>GPSEGIVPGPPTDLSVTEATRSYVVLSWKPPGQRGHEGIMYFVEKCEAGTENWQRVNTELPVKSPRFALFDLAEGKSYCF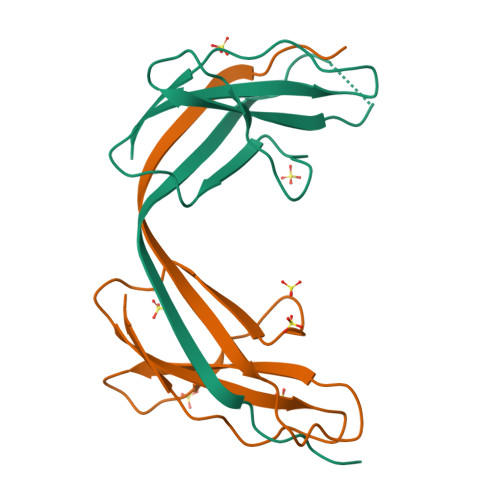RVRCSNSAGVGEPSEATEVTVVGDK[2x]>EANGNQDIAKLEAYFGTKMEMTLKDLPTVGVHTPSPWAGPYWPTYQDSINVQWSQGQPSAAEKYAKAFGKDVKTFMDAVSKKNGIDSQSGRKKCSSDDDCSTLTDGSSCSIRTGKTSGYCIPTWFGISHAWSPAAILETEPKCPVKHNGVTFQPMDLKALVSLVYDGARVQTVFTGARFNGGTDTTDEYGRHSNNAYRDLNPAYFHIASANILGKLNSTFVADVTAGAEVWNQPVRGFKVYEQTEMTLE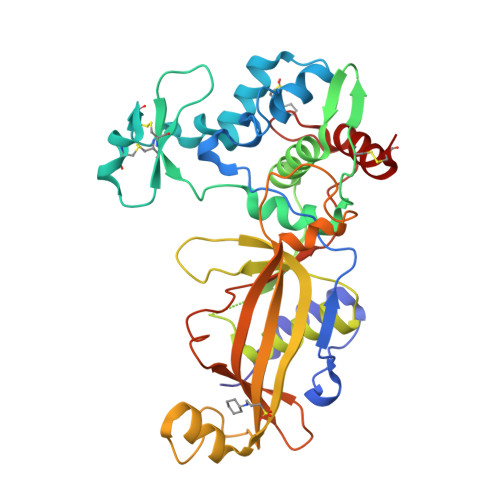EGAQTFYGLEAYPWNAAAKSLVYVKSRLSWIYETYTDGGLVSSGQIDKFTTGQYYYYLLELDDAGEIIGGEWVYGSDDDHPDFLWLPKAKPAANTVTSVGLSYADVSMLLKKSAACTA[2x]> MERTELLKPRTLADLIRILHELFAGDEVNVEEVQAVLEAYESNPADWALYAKFDQYRYTRNLVDQGNGKFNLMILCWGEGHGSSIHDHTDSHCFLKLLQGNLKETLFDWPDKKSN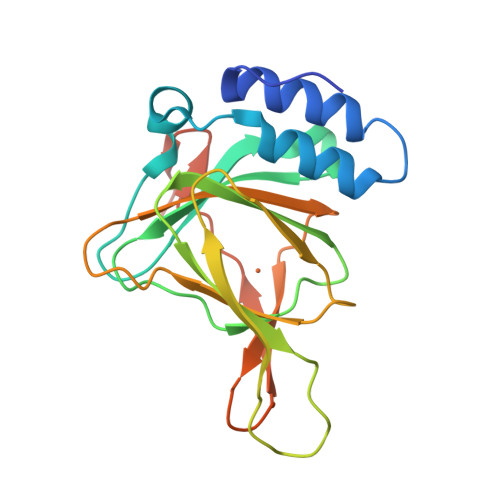EMIKKSERTLRENQCAYINDSIGLHRVENVSHTEPAVSLHLYSPPFDTCHAFDQRTGHKNKVTMTFHSKFGIRTPFTTSGSLENN> AKCVSYGVAQIKAPALHSQGYTGSNVKVAVLDSGIDSSHPDLNVAGGASFVPSETNPFQDNNSHGTHVAGTVLAVAPSASLYAVKVLGADGSGQYSWVINGIEWAIANNMDVINMSLGGPSGSAALKAAVDKAVASGVVVVAAAGNSGTSGSSSTVSYPAKYPSVIAVGAVDSSNQRAPFSSVGPELDVMAPGVSICSTLPGGKYGAHSGTCPASNHVAGAAALILSKHPNWTNTQVRSSLENTATKLGDSFYYGKGLINVEAAAQHHHHHH

Omniligase-1 is a broadly applicable enzyme for peptide bond formation between an activated acyl donor peptide and a non-protected acyl acceptor peptide. The enzyme is derived from an earlier subtilisin variant called peptiligase by several rounds of protein engineering aimed at increasing synthetic yields and substrate range. Mutation A225N in the S1′ pocket and F189W of the S2′ pocket increased the synthesis to hydrolysis (S/H) ratio and overall coupling efficiency, whereas the I107V mutation was added to S4 pocket to increase the reaction rate. The final omniligase variants appeared to have a very broad substrate range, coupling more than 250 peptides in a 400-member library of acyl acceptors, as indicated by a high-throughput FRET assay.

Despite extensive screening of thousands of conditions, Oml-1 itself refused to form crystals. The crystal of Pre-6, that differs from Oml-1 by the single point mutation W189F, was grown in crystal form B, identical to Pre-3, with the same crystallization agent, polyacrylic acid. Among other single point mutations in the omniligase variants only I107V effects the substrate binding pockets and reaction rates by enlarging the hydrophobic S4 subsite with one methyl group. All conditions giving crystals in this study were employed for crystallization attempts of Oml-1 but without success. Therefore, an omniligase-1 model was constructed by superimposing the sidechain W189 of crystal form C (Pre-4 and Pre-5) on Pre-6. This model was used for later studies (see below).>[2x]MRYGHFDDEAREYVITTPHTPYPWINYLGSEQFFSLLSHQAGGY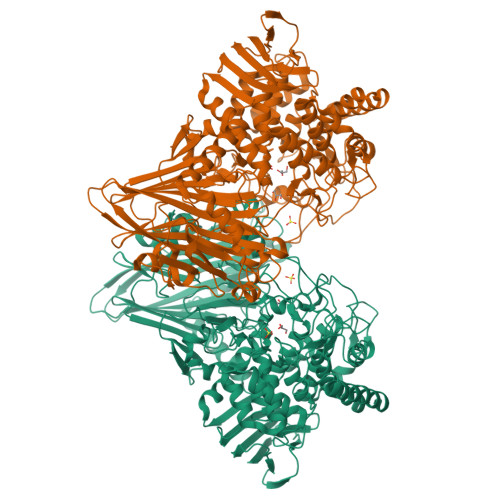SFYRDAKMRRLTRYRYNNIPADAGGRYLYVNDGGDVWTPSWLPVKADLDHFEARHGLGYSTITGERNGVRVETLFFVPVGENAEVQKVTVTNTSDSYKSLTLFSFVEFCLWNAQDDQTNYQRNLSIGEVEVEQESPHGSAIYHRTEYRERRDHYAVFAVNTQAEGFDTDRDTFVGAYNSLGEAAVPLKGESANSVASGWYPIGSHSVAVSLAPGESRELVYVLGYVENPDEEKWADDAKQVVNKERAHALLSRFATSEQTDAAFAALKDYWTDLLSTYSVSSNDEKLDRMVNIWNQYQCMVTFNMSRSASFFETGIGRGMGFRDSNQDLLGFVHLIPERARERIIDIASTQFADGSAYHQYQPLTKRGNNDIGSGFNDDPLWLIAGTAAYIKETGDFSILDEPVPFDNEPGSEVPLFEHLTRSFEFTVTHRGPHGLPLIGRADWNDCLNLNCFSTTPGESFQTTENQAGGVAESTFIAAQFVLYGEQYAELAARRGLADVADRARGHVAEMRDALLTDGWDGSWFLRAYDYYGNPIGTDAHDEGKIWIEPQGFAVMAGVGVGEGPQDTDAPAIKALDSVNEMLATDHGMVLQYPAYTTYQVHMGEVSTYPPGYKENGGIFCHNNPWVIIAETVVGRGGRAFDYYKRITPAYREDISDVHRLEPYVYAQMIAGKEAVRHGEAKNSWLTGTAAWNFVTVSQYLLGVRPEYDGLVVDPQIGPDVPSFTVTRVARGATYEITVTNSGTDGSRGRLVVDGTPVEGNLVPYAPAGSTVRVDVTL>SVVIVGKISFCPKDVLGHGAEGTIVYRGMFDNRDVAVKRILPECFSFADREVQLLRESDEHPNVIRYFCTEKDRQFQYIAIELCAATLQEYVEQKDFAHLGLEPITLLQQTTSGLAHLHSLNIVHRDLKPHNILISMPNAHGKIKAMISDFGLCKKLAVGRHSFSRRSGVPGTEGWIAPEMLSEDCKENPTYTVDIFSAGCVFYYVISEGSHPFGKSLQRQANILLGACSLDCLHPEKHEDVIARELIEKMIAMDPQKRPSAKHVLKHPFFWSLEKQLQFFQDV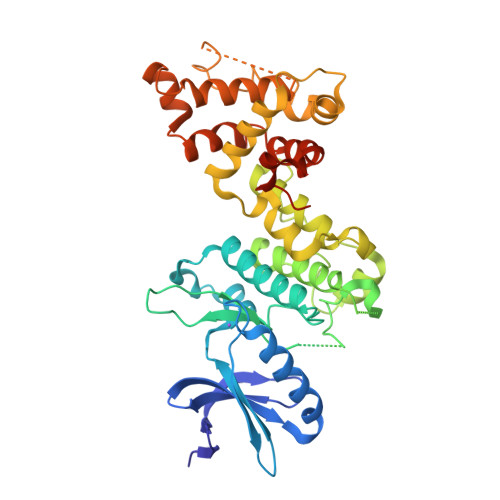SDRIEKESLDGPIVKQLERGGRAVVKMDWRENITVPLQTDLRKFRTYKGGSVRDLLRAMRNKKHHYRELPAEVRETLGSLPDDFVCYFTSRFPHLLAHTYRAMELCSHERLFQPYYFHEPPEPQPPVTPDAL[2x]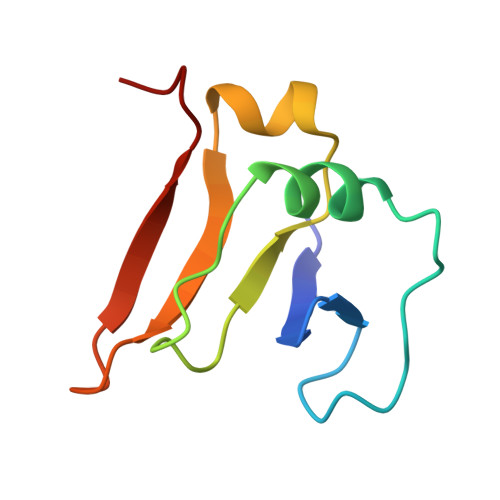> MRALFYKDGKLFTDNNFLNPVSDDNPAYEVLQHVKIPTHLTDVVVYEQTWEEALTRLIFVGSDSKGRRQYFYGKMHV>MAHHHHHHHRSTPLPLVRRVPTGQVITQCTTPNTIALTFDDGPSEYTPQLLDLLSRYSARATFFVLGDAAAQNPGLLQRMRDEGHQVGAHTYDHVSLPSLGYDGIASQMTRLEEVIRPALGVAPAYMRPPYLETNELVLQVMRDLDYRVISASVDTKDYENQDADAIINTSFQLF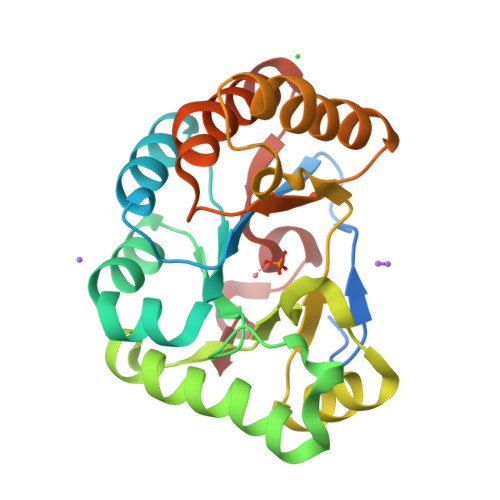LDQLDAGGNIVLAHDIHYWTVASLAERMLQEVNARGLIATTVGDCLGDGEIAWYH[2x]> GLFDAPGRSQFVPADQAFAFDFQQNQHDLNLTWQIKDGYYLYRKQIRITPEHAKIADVQLPQGVWHEDEFYGKSEIYRDRLTLPVTINQASAGATLTVTYQGSADAGFCYPPETKTVPLSEVVANNAAPQPVSVPQQE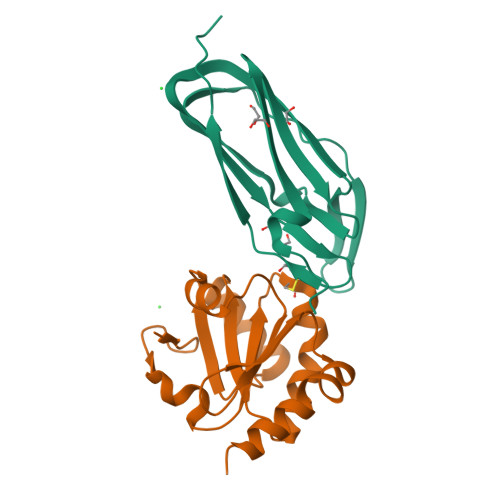QPTAQ;> KPVPKFRLESLDNPGQFYQADVLTQGKPVLLNVWATWCPTSRAEHQYLNQLSAQGIRVVGMNYKDDRQKAISWLKELGNPYALSLFDGDGMLGLDLGVYGAPETFLIDGNGIIRYRHAGDLNPRVWEEEIKPLWEKYSKEAAQHHHHHH>MNYPAEPFRIKSVETVSMIPRDERLKKMQEAGYNTFLLNSKDIYIDLLTDSGTNAMSDKQWAGMMMGDEAYAGSENFYHLERTVQELFGFKHIVPTHQGRGAENLLSQLAIKPGQYVAGNMYFTTTRYHQEKNGAVFVDIVRDEAHDAGLNIAFKGDIDLKKLQKLIDEKGAENIAYICLAVTVNLAGGQPVSMANMRAVRELTAAHGIKVFYDATRCVENAYFIKEQEQGFENKSIAEIVHEMFSYADGCTMSGKKDCLVNIGGFLCMNDDEMFSSAKELVVVYEGMPSYGGLAGRDMEAMAIGLREAMQYEYIEHRVKQVRYLGDKLKAAGVPIVEPVGGHAVFLDARRFCEHLTQDEFPAQSLAASIYVETGVRSAERGIISA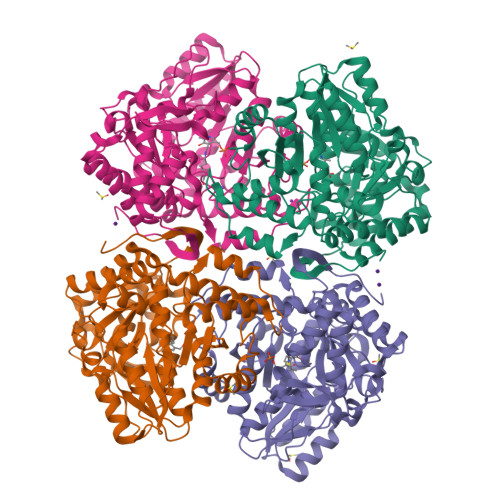GRNNVTGEHHRPKLETVRLTIPRRVYTYAHMDVVADGIIKLYQHKEDIRGLKFIYEPKQLRFFTARFDYI[4x]2'-azidocytidine | C9 H13 N6 O4 | 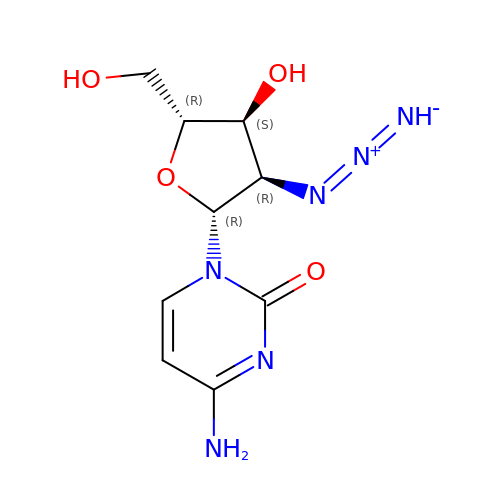SXKUZFQHWHCRFO-XVFCMESISA-N> ARRKREHSTLWFPE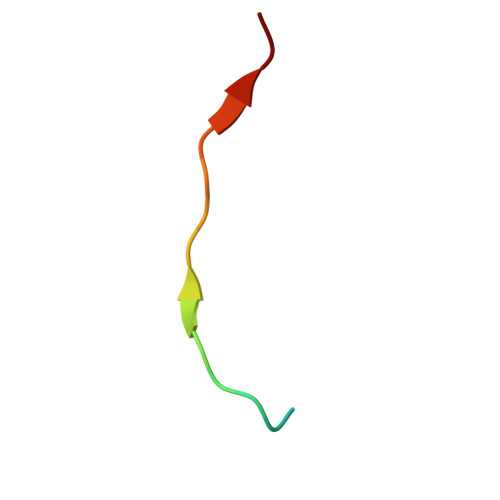GFSL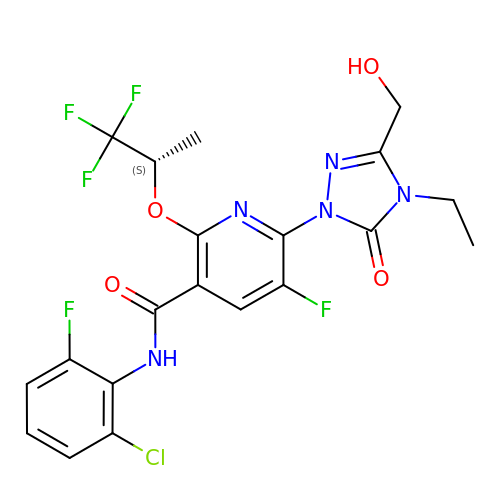(6M)-N-(2-chloro-6-fluorophenyl)-6-[4-ethyl-3-(hydroxymethyl)-5-oxo-4,5-dihydro-1H-1,2,4-triazol-1-yl]-5-fluoro-2-{[(2S)-1,1,1-trifluoropropan-2-yl]oxy}pyridine-3-carboxamide | C20 H17 Cl F5 N5 O4 | OTVJNMGRFHZVRL-VIFPVBQESA-N>GPLGSMDAATLTYDTLRFAEFEDFPETSEPVWILGRKYSIFTEKDEILSDVASRLWFTYRKNFPAIGGTGPTSDTGWGCMLRCGQMIFAQALVCRHLGRDWRWTQRKRQPDSYFSVLNAFIDRKDSYYSIHQIAQMGVGEGKSIGQWYGPNTVAQVLKKLAVFDTWSSLAVHIAMDNTVVMEEIRRLCRTSVPCAGATAFPADSDRHCNGFPAGAEVTNRPSPWRPLVLLIPLRLGLTDINEAYVETLKHCFMMPQSLGVIGGKPNSAHYFIGYVGEELIYLDPHTTQPAVEPTDGCFIPDESFHCQHPPCRMSIAELDPSIAVGFFCKTEDDFNDWCQQVKKLSLLGGALPMFELVEQQPSHLACPDVLNLSLDSSDVERLERFFDSED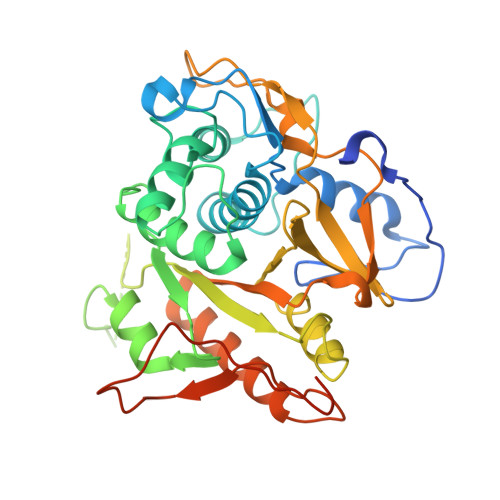EDFEILSL[2x]> MRGSRSGHGNGGGNSNSGGGSNSSV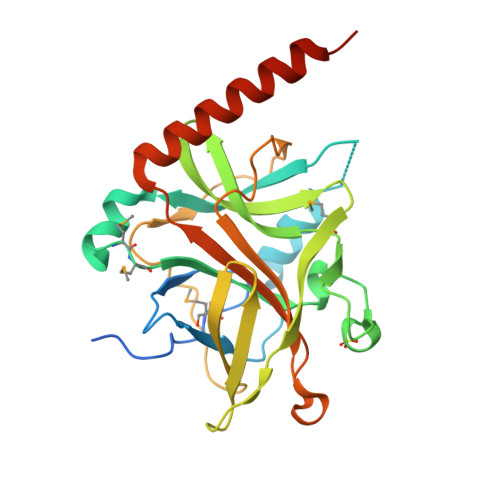AAPMAFGFPALAAPGAGTLGISVSGEALSAAIADIFAALKGPFKFSAWGIALYGILPSEIAKDDPNMMSKIVTSLPAETVTNVQVSTLPLDQATVSVTKRVTDVVKDTRQHIAVVAGVPMSVPVVNAKPTRTPGVFHASFPGVPSLTVSTVKGLPVSTTLPRGITEDKGRTAVPAGFTFGGGSHEAVIRFPKESGQKPVYVSVTDVLTPAQVKQRQDEEKRLQQEWNDAHPVEVAERRS Janus kinases (Jaks) have broad roles in immune regulation via their action in cytokine signalling. These non-receptor tyrosine kinases phosphorylate receptor chains, which in turn recruit and phosphorylate members of the Signal Transducer and Activator of Transcription (STAT) family. Tyk2 functions together with Jak2 in the signaling of IL-12 and IL-23 via its interaction with the IL-12Rβ1 receptor chain, and in the coordinated phosphorylation of STAT3 & STAT4. Here we present the first mouse Tyk2 crystal structures, which are complexed to 3-aminoindazole compounds.

We also present the structure of Compound 2 complexed to mouse Tyk2, which was solved using inhibitor soaking methods. The placement of this moiety is guided by the sulfonamide linkage’s stabilizing interactions with the NH backbone of Glu898 in the glycine-rich loop, and conserved residues Asn1021 and Arg1020. The structure of Tyk2 and Compound 2 is illustrated in Figure 5b. The binding mode and trajectory of the chlorophenyl is identical to that of Compound 1 and, as a result, the glycine-rich loop adopts the same conformation in both structures. The furan substituent on the hinge-binding 3-aminoindazole core was well-ordered, providing clear evidence that the inhibitor soak was successful. The furan occupies the extended hinge region, sandwiched between Arg894 and Gly977. In the mouse Tyk2 structures, complexed to either Compound 1 or Compound 2, the steric bulk of the sulfonamide chlorophenyl moiety occupies substantial hydrophobic space under the glycine-rich loop and would potentially disrupt the His/Asp “glycine-rich loop lock,” thereby creating a larger active site pocket. Compound 2 (30 μM) significantly increased resistance to partial proteolysis by thermolysin. However, the rate of degradation of the enzyme to smaller forms (<27 kDa) is reduced by 13-fold. Like all protein kinases, the ATP binding site for Tyk2 is nestled between the N-terminal and C-terminal lobes. Our proteolysis data suggest that the conformational flexibility of the kinase, other than a ~2 kDa portion of one terminus (likely the N-terminus based on the disorder seen from residue 870–884 in the crystal structure described below), is decreased by the binding of these 3-aminoindazole inhibitors. We obtained crystals with a kinase-inactive form of the mouse Tyk2 catalytic domain, only in the presence of an ATP-competitive 3-aminoindazole inhibitor. This crystal form provided a robust inhibitor soaking platform that enabled structure-based drug design of Jak inhibitors.

> SDPTVFHKRYLKKIRDLGEGHFGKVSLYCYDPTNDGTGEMVAVKALKEGCGPQLRSGWQREIEILRTLYHEHIVKYKGCCEDQGEKSVQLVMEYVPLGSLRDYLPRHCVGLAQLLLFAQQICEGMAYLHAQHYIHRALAARNVLLDNDRLVKIGDFGLAKAVPEGHEYYRVREDGDSPVFWYAPECLKECKFYYASDVWSFGVTLYELLTYCDSNQSPHTKFTELIGHTQGQMTVLRLTELLERGERLPRPDRCPCEIYHLMKNCWETEASFRPTFQNLVPILQTAQEKYQ>[12x]MPRSLANAPIMILNGPNLNLLGQRQPEIYGSDTLADVEALCVKAAAAHGGTVDFRQSNHEGELVDWIHEARLNHCGIVINPAAYSHTS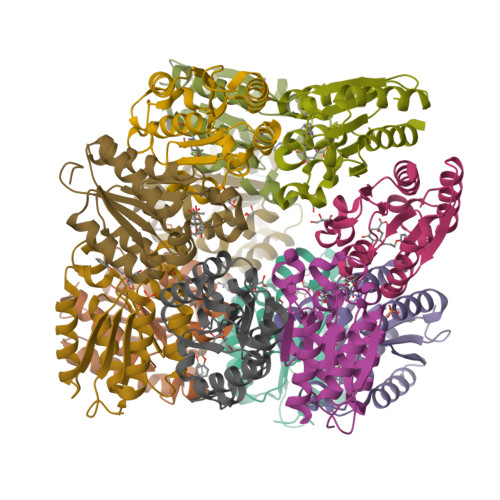VAILDALNTCDGLPVVEVHISNIHQREPFRHHSYVSQRADGVVAGCGVQGYVFGVERIAALAGAGSARA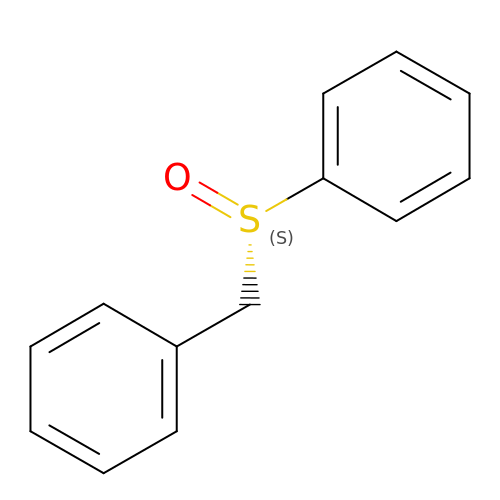phenylsulfinylmethylbenzene | C13 H12 O S | FBPGAWABXWMRAR-HNNXBMFYSA-N> MQQIDLNVTCRYAGVFHVEKNGRYSISRTEAADLCQAFNSTLPTMDQMKLALSKGFETC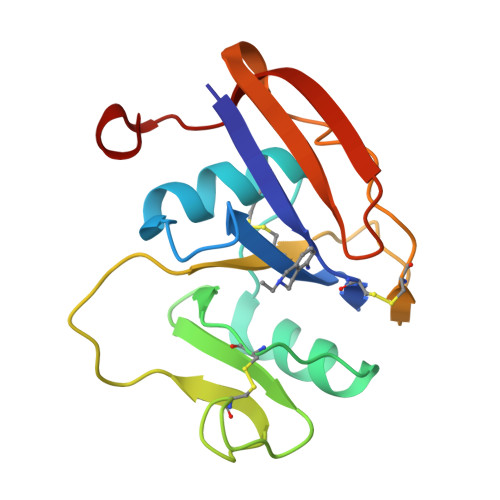RYGFIEGNVVIPRIHPNAICAANHTGVYILVTSNTSHYDTYCFNASAPPEEDCTSVTDLPNSFDGPVTITIVNRDGTRASKKGEYRTHQEDI Type III PKS catalysis involves the loading of a CoA-tethered substrate onto an active-site cysteine followed by chain elongation via iterative decarboxylative Claisen condensations of malonyl-CoA. Linear poly­ketide intermediates undergo a terminal intramolecular cyclization reaction to produce the final cyclic polyketide product. The five-layered αβαβα topology of secondary-structural elements of each monomer is consistent with the ‘thiolase fold’ originally observed in thiolase and present in all known structures of type III PKSs.

Biphenyl synthase (BIS) generates the core chemical scaffolds of biphenyl and dibenzofuran phytoalexins commonly found in the Pyrinae subtribe (Rosaceae; Liu et al., 2007; Khalil et al., 2013). Additionally, each monomer of MdBIS3 contained electron density consistent with 1,3-butanediol, the cryoprotectant. Despite the use of reducing agents in all buffers and crystallization solutions, the electron-density maps indicated that the active-site cysteines of the MdBIS3 crystals were oxidized to their sulfinic acid derivatives (–SO2H). Differences in the side-chain torsion angles of Tyr260 in MdBIS3 (χ1 = 61°) and Tyr269 in HaBPS (χ1 = 50°) compared with Phe265 of CHS (χ1 = 170°) significantly reorient the tyrosine side chains and increase the conformational flexibility of the nearby Leu262 in MdBIS3 and Leu271 in HaBPS. Lastly, the side-chain conformation of Tyr260 in MdBIS3 is stabilized via the presence of a water-mediated hydrogen bond to the backbone carbonyl of Phe192. Replacement of Thr197 in CHS with Phe in MdBIS3 (Phe192) appears to be responsible for closing off access to the coumaroyl-binding region of CHS. Met267 of HaBPS is substituted with a Phe in MdBIS3 (Phe258) and seems to primarily function in stabilizing the conformation of nearby residues including Phe192. The sides of this novel pocket in MdBIS3 are formed from the side chains of Cys125, Ala127, Ala157, Glu187 and Ala336 as well as the main-chain atoms of Gly158, Ala157, Gly335 and Ala336. Additionally, the novel pocket of MdBIS3 contains ordered waters that could function similar to the nucleophilic water that is essential for the aldol switch of stilbene synthases.

>GSMAPLVKNEPQHAKILAIGTANPPNVYHQKDYPDFLFRVTKNEHRTDLREKFDRICEKSRTKKRYLHLTEEMLKANPNIYTYGAPSLDVRQDICNIEVPKLGQEAALKAIKEWGQPISRITHLIFCTASCVDMPGCDFQLIKLLGLDPSVTRTMIYEAGCYAGATVLRMAKDFAENNKGARVLVVCAEITTVFFHGLTDTHLDILVGQALFADGASAVIVGANPEPEIERPLFEIVACRQTILPNSEHGVVANIREMGFNYYLSGDVPKFVGGNVVDFMTKTFEKVDGKKKDWNSLFFSVHPGGPAIVDQVEEKLGLKEGKLRATRHVLSEYGNMGAPTVHFILDEMRNKSIEEGKTTTGEGLEWGVVIGIGPGLTVETAVLRSESIRC[2x]> GVTTLLSYLASESEGSLKVQGWSASGGRAEVVSDAEGTGGKAVKLTKEAGKSSWVLEYAAGNG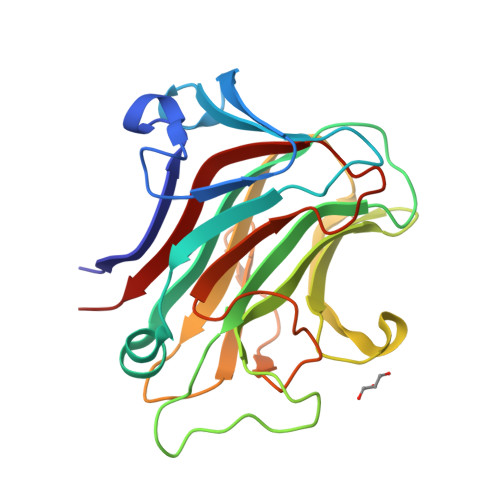AALLQKGGQIRCRFKVSGALAANQYVMAFYWPVSSLPQGVALTGDGGNNLLAAFYIQTDAKDLNVMYHNAKVATNNLKLGTFGAFDNEWHTLAFRFAGNNSLQVTPVIDGQDGTPFTLTQSPVSAFAADKLHVTDITRGATYPVLIDSIAVEVNS> DPVQNSCDNCQPGTFCRKYNPVCKSCPPSTFSSIGGQPNCNICRVCAGYFRFKKFCSSTHNAECECIEGFHCLGPQCTRCEKDCRPGQELTKQGCKTCSLGTFNDQNGTGVCRPWTNCSLDGRSVLKTGTTEKDVV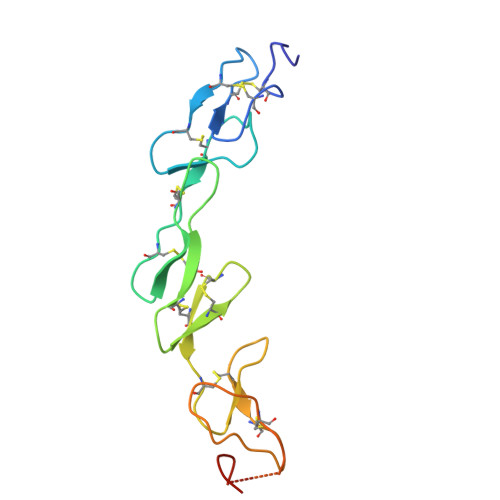CGP>MSYQVLARKWRPQTFADVVGQEHVLTALANGLSLGRIHHAYLFSGTRGVGKTSIARLLAKGLNCETGITATPCGVCDNCREIEQGRFVDLIEIDAASRTKVEDTRDLLDNVQYAPARGRFKVYLIDEVHMLSRHSFNALLKTLEEPPEHVKFLLATTDPQKLPVTILSRCLQFHLKALDVEQIRHQLEHILNEEHIAHEPRALQLLARAAEGSLRDALSLTDQAIASGDGQVSTQAVSAMLGTLDDDQALSLVEAMVEANGERVMALINEAAARGIEWEALLVEMLGLLHRIAMVQLSPAALGNDMAAIELRMRELARTIPPTDIQLYYQTLLIGRKELPYAPDRRMGVEMTLLRALAFHPRMPLPEPEVPRQ[3x];> MIRLYPEQLRAQLNEGLRAAYLLLGNDPLLLQESQDAVRQVAAAQGFEEHHTFSIDPNTDWNAIFSLCQAMSLFASRQTLLLLLPENGPNAAINEQLLTLTGLLHDDLLLIVRGNKLSKAQENAAWFTALANRSVQVTCQTPEQAQLPRWVAARAKQLNLELDDAANQVLCYCYEGNLLALAQALERLSLLWPDGKLTLPRVEQAVNDAAHFTPFHWVDALLMGKSKRALHILQQLRLEGSEPVILLRTLQRELLLLVNLKRQSAHTPLRALFDKHRVWQNRRGMMGEALNRLSQTQLRQAVQLLTRTELTLKQDYGQSVWAELEGLSLLLCHKPLADVFIDG;> MRWYPWLRPDFEKLVASYQAGRGHHALLIQALPGMGDDALIYALSRYLLCQQPQGHKSCGHCRGCQLMQAGTHPDYYTLAPEKGKNTLGVDAVREVTEKLNEHARLGGAKVVWVTDAALLTDAAANALLKTLEEPPAETWFFLATREPERLLATLRSRCRLHYLAPPPEQYAVTWLSREVTMSQDALLAALRLSAGSPGAALALFQGDNWQARETLCQALAYSVPSGDWYSLLAALNHEQAPARLHWLATLLMDALKRHHGAAQVTNVDVPGLVAELANHLSPSRLQAILGDVCHIREQLMSVTGINRELLITDL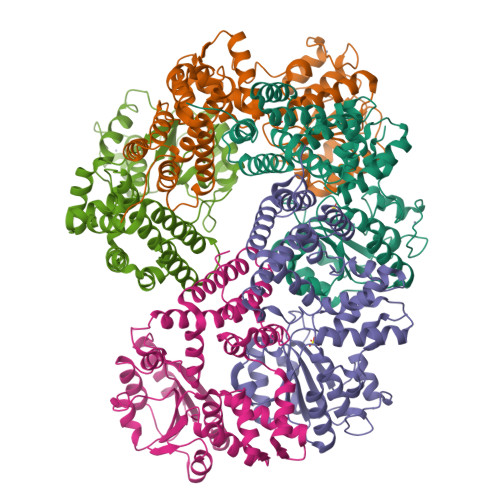LLRIEHYLQPGVVLPVPHL>[3x]MGAKLAKTLQRFENKIKAGDYYEAHQTLRTIANRYVRSKSYEHAIELISQGALSFLKAKQGGSGTDLIFYLLEVYDLAEVKVDDISVARLVRLIAELDPSEPNLKDVIT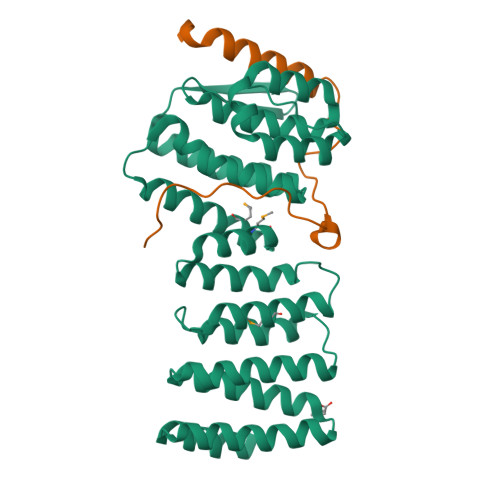GMNNWSIKFSEYKFGDPYLHNTIGSKLLEGDFVYEAERYFMLGTHDSMIKYVDLLWDWLCQVDDIEDSTVAEFFSRLVFNYLFISNISFAHESKDIFLERFIEKFHPKYEKIDKNGYEIVFFEDYSDLNFLQLLLITCQTKDKSYFLNLKNHYLDFSQAYKSELEFLGQEYFNIVAPKQTNFL;>TSASGPEHEFVSKFLTLATLTEPKLPKSYTKPLKDVTNLGVPLPTLKYKYKQNR[3x]>[2x]MTIRSAEHATLVIERHLKAPIARVFRAWSAPEAKRQWFACHGEWQALDYGLDFR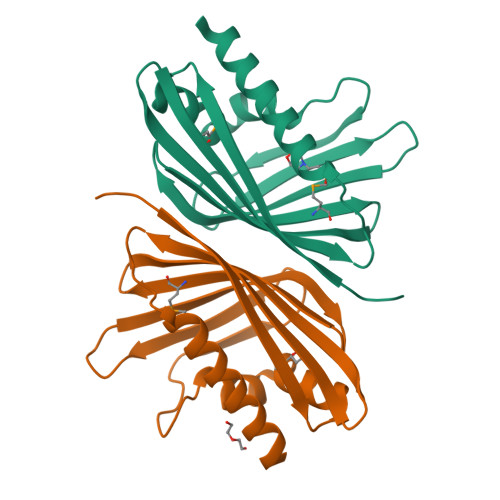PGGTERNYVADTDGLLHAYDAHYIDIVPNARIIYAYEMKLGETRISASLTTVAFEAEPGGTKMVFTEQVVFLDGYADNGARLQGTEIGLDNLELFLEREESPIH(4S)-4-(2-AMINO-6-PHENOXYQUINAZOLIN-3(4H)-YL)-N,4-DICYCLOHEXYL-N-METHYLBUTANAMIDE 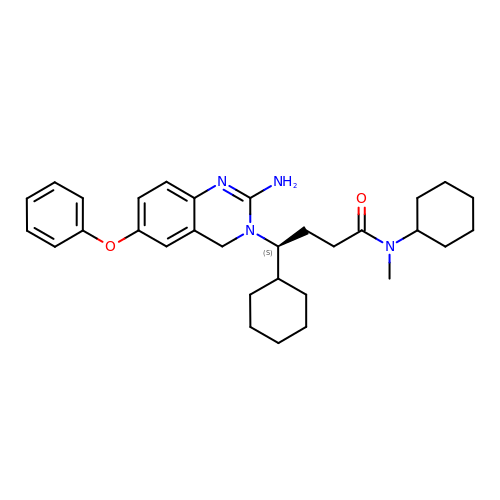| C31 H42 N4 O2 | JKQCQYBXDQPJNC-LJAQVGFWSA-N> MLPNTELYNTIFSETRKFTRESFKEIEHLTAKLANDRVARHDFLFNNSIALISDYSGEDSNGNQLQATVTIPNEITNPKEYDPSDYPLAEDESFFKQGHKYDYLVTFRAGSLTNTYEPKTKMYKLHAALDKLMHVKQRKSRFADLWRELCAVIASLDVWYQTTNYPLRTYVKLLFHKGDEFPFYESPSQDKIIFNDKSVASILPTFVYTCCQVGTAIMSGILTHVESIVAMNHFLHCAKDSYIDEKLKIKGIGRSWYQEALHNVGRATVPVWSQFNEVIGHRTKTTSEPHFVSSTFISLRAKRAELLYPEFNEYINRALRLSKT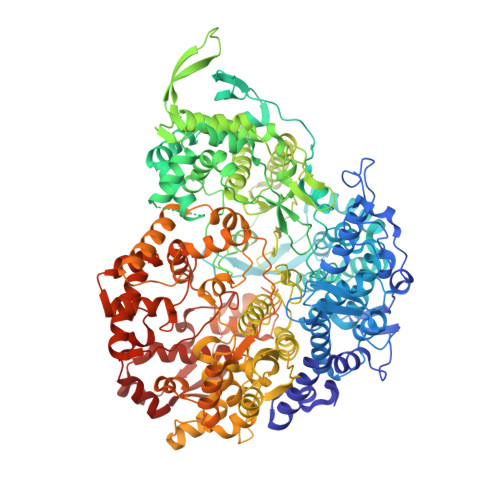QNDVANYYAACRAMTNDGTFLATLTELSLDAAVFPRIEQRLVTRPAVLMSNTRHESLKQKYANGVGSIAQSYLSSFTDEIAKRVNGIHHDEAWLNFLTTSSPGRKLTEIEKLEVGGDVAAWSNSRIVMQAVFAREYRTPERIFKSLKAPIKLVERQQSDRRQRAISGLDNDRLFLSFMPYTIGKQIYDLNDNAAQGKQAGNAFDIGEMLYWTSQRNVLLSSIDVAGMDASVTTNTKDIYNTFVLDVASKCTVPRFGPYYAKNMEVFEVGKRQSQVKYVNAAWQACALEAANSQTSTSYESEIFGQVKNAEGTYPSGRADTSTHHTVLLQGLVRGNELKRASDGKNSCLTTIKILGDDIMEIFQGNENDTHDHAVSNASILNESGFATTAELSQNSIVLLQQLVVNGTFWGFADRISLWTREDTKDIGRLNLAMMELNALIDDLLFRVRRPEGLKMLGFFCGAICLRRFTLSVDNKLYDSTYNNLSKYMTLVKYDKNPDFDSTLMSLILPLAWLFMPRGGEYPAYPFERRDGTFTEDESMFTARGAYKRRLLYDVSNIREMIQQNSMVLDDDLLHEYGFTGALLLIDLNILDLIDEVKKEDISPVKVNELATSLEQLGKLGEREKSRRAASDLKIRGHALSNDIVYGYGLQEKIQKSAMATKETTVQSKRVSSRLHEVIVAKTRDYKIPTMPADALHLYEFEVEDVTVDLLPHAKHTSYSNLAYNMSFGSDGWFAFALLGGLDRSANLLRLDVASIRGNYHKFSYDDPVFKQGYKIYKSDATLLNDFFVAISAGPKEQGILLRAFAYYSLYGNVEYHYVLSPRQLFFLSDNPVSAERLVRIPPSYYVSTQCRALYNIFSYLHILRSITSNQGKRLGMVLHPGLIAYVRGTSQGAILPEADNV> GSHMVPDTPTRLVFSALGPTSLRVSWQEPRCERPLQGYSVEYQLLNGGELHRLNIPNPAQTSVVVEDLLPNHSYVFRVRAQSQEGWGREREGVITIESQVHPQSPLCPLPGSAFTLSTPSAPGP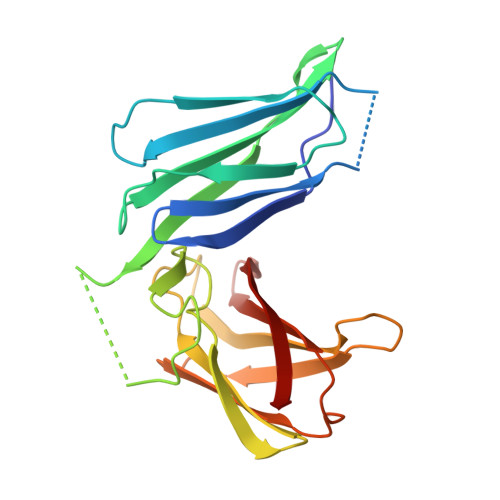LVFTALSPDSLQLSWERPRRPNGDIVGYLVTCEMAQGGGPATAFRVDGDSPESRLTVPGLSENVPYKFKVQARTTEGFGPEREGIIRIES2-(1H-indol-3-yl)-N-[(1-methyl-1H-pyrrol-2-yl)methyl]ethanamine 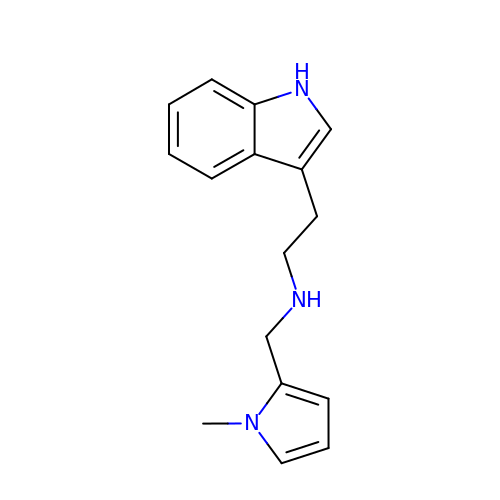| C16 H19 N3 | JMDFJNUSALBEDM-UHFFFAOYSA-N AChBPs are homopentameric, water-soluble homologs of the ligand-binding domain of LGICs and well-established structural surrogates for nicotinic acetylcholine receptors (nAChR). Importantly, AChBPs can bind nAChR-specific ligands and induce similar conformational changes as in the membrane bound receptors. LGICs are activated by ligands binding at subunit interfaces of their extracellular domains, thereby inducing conformational changes that affect the structure of a central pore and its ability to transport ions through the membrane. Additional density was found in all structures at the interface between the subunits in the orthosteric agonist and antagonist binding site, next to loop C in which the respective ligands could be modelled.

The sensorgrams had concentration dependent distortions in both the association and dissociation phases, with a negative slope at steady state and signals below baseline once the ligand injection was stopped. Surface Acoustic Wave (SAW) biosensor technology was used to confirm that distortions observed in SPR biosensor data for interactions between compounds VUF6105, VUF22430, and VUF24234, and AChBP indeed result from ligand-induced conformational changes. The three VUF compounds resulted in significant ΔSHG responses with all labelling variants, with VUF22430 giving very high signals. Similarly, VUF6105 resulted in a significant compaction, while VUF24234 resulted in an expansion. As seen from the different conformational changes induced by each compound, this analysis revealed that the binding modes of VUF6105 and VUF24234 are different. The unit cell was comprised of two or four pentamers of Ls-AChBP in the presence of FL1613, FL1856, FL1888, FL3044, VUF24234 and VUF6105. Notably, binding of FL1888, VUF24234 and VUF6105 results in a movement of the loop closer to the compound, while binding of FL1856, FL3044, FL1613 and FL1909 does not have the same effect. The violin plot revealed that conformational changes in loop C occurred to a higher degree in the AChBP structures with compounds FL1888, VUF24234 and VUF6105 than in the other structures. This correlated with the results from the SPR, SAW and SHG biosensor experiments, which all indicated conformational changes in AChBP upon binding of these compounds.

>[10x]LDRADILYNIRQTSRPDVIPTQRDRPVAVSVSLKFINILEVNEITNEVDVVFWQQTTWSDRTLAWNSSHSPDQVSVPISSLWVPDLAAYNAISKPEVLTPQLARVVSDGEVLYMPSIRQRFSCDVSGVDTESGATCRIKIGSWTHHSREISVDPTTENSDDSEYFSQYSRFEILDVTQKKNSVTYSCCPEAYEDVEVSLNFRKKGR>MSTAGDGERGTVGQEDSAAARPFRFSPEPTLEDIRRLHAEFAAERDWEQFHQPRNLLLALVGEVGELAELFQWKSDTEPGPQAWPPKERAALQEELSDVLIYLVALAARCHVDLPQAVISKMDTNRQRYPVH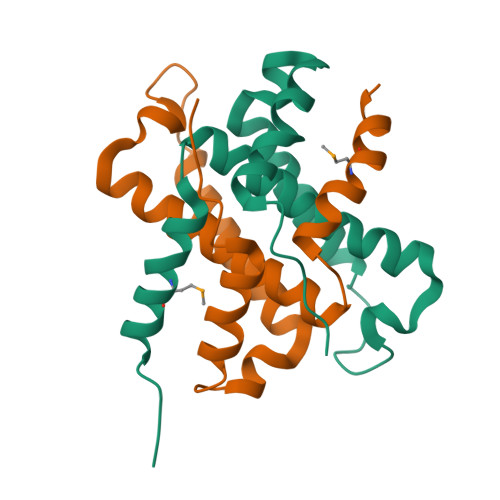LSRGSACKYTDLPRGTISENQAVGAGDPASELRDQAST[2x]> MKQGFARPTPERAPVVKPENIVLPTPLSVPPPEGKPWWLVVVGVLVVGLLVGMVGMTVASGSRLFLGAGAIFPIFMIGGVAMMMFGGRFGGQQQMSRPKLDAMRAQFMLMLDMLRETAQESADSMDANYRWFHPAPTTLAAAVGSSRMWERQPDGKDLNFGVVRVGVGMTRPEVTWGEPQNMPTDIELEPVTGKALQEFGRYQSVVYNLPKMVSLLVEPWYSLVGEREQVLGLTRAIICQLAFSHGPDHVQMIVVTSDPDRWDWVKWIPHFGDPRRRDAAGNARMVYTSVREFATEQAELFAGRGSFTPRHASSSAETPTPHHVIISDIEDPQWEYVISSEGVDGVTFFDLTGSPLWTGAPQRVLRFTDSAGVIETLPRDRDTWMVIDDNAWFFALADQMSEADAEQFAHQMAHWRLAEAYEEIGQRVVQLGARDILSYYGIDDAGEIDFNTLWSGSGRRDLLSRSRLRIPFGNRADNGELLFLDMKSLDEGGDGPHGVMSGTTGSGKSSLVRTVIASLMLAHPPEELQFVLADLKGGSAVKPFDGVPHVSRIITDLEDDQALMERFLEAMWGEIARRKEICFSAGVDGAKEYNELRARMKARGEDMPPLPMLVVVIDEFYEWFRIMPTAVDVLDSIGRQGRAYWVHLMMASQTIESRAEKLMENMGYRLVLKAQTAGAAQAAGVPNAVNLPSQAGLGYFRKSGDEIIRFQAEYLWRDYRRGSSYDGEEQAPLTHSVDYIRPQLFTTAFAPLEVSVSGPDGQSALPQVVDGEAVNGHRGGDDVDEEEEALRTPKVGTVIIDQLRQIDFEPYRLWHPPLDVPVPIDELVNRFLGRPWQQDYGTAKNLVFPIGIIDRPYKHDQPPWTVDTSGAGANVLILGAGGAGKTTALQTLICAAALTHTPEQVQFYCLAYSGTALTTVANLPHVGGVSGPTDPYGVRRTVAEVLGLVRDRKRSFLEYDVPSMEVFRRRKFGGEPGGVPDDGFGDVYLVIDNYRALAEENEVLIEQVNQIINQGPSFGVHVVATADRESELRPPVRSGFGSRVELRLAAVEDAKLVRSRFAKDVPPKPGRGMVAVNYVRLDSDPQAGLHTLVARPALGSTPDAVFESDSVAAAVRQVAAGEARPVRRLPARFGLDQLRQVAAADRRQGVGAGGIAWAISELDLQPVYLN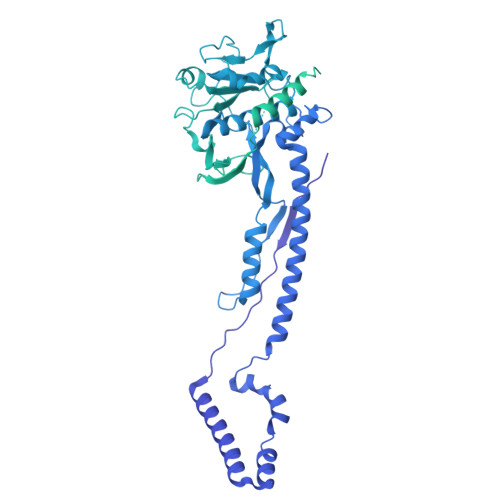FADNAHLMVTGRRECGRTTTLATIMSEIGRIYAPGASTAPPTSRPSAQVWLVDPRRQLLTVLGSDYVEKFAYNLDGVAAMMDDLAAALARREPPPGLSAEELLSRSWWSGPEIFLIIDDIQQLPPGFDSPLHKAAPWVTRAADVGLHVFVTRTFGGWSSAGSDPILRALHQANAPLLVMDADPDEGFIRGKMKGGPLPRGRGLLMAEDTGVFVQVAATDLRR> SPNVEACGYSDRVQQITLGNSTITTQEARNAIVCYAEWPEYLSDNDASDVNKTSKPDISVCRFYTLDSKTWKATSKGWCWKLPDALKDMGVFGQNMFYHSLGRTGYTIHVQCNATKFHSGCLLVVVIPEHQLASHEGGTVSVKYKYTHPGDRGIDLDTVEVAGGPTSDAIYNMDGTLLGNLLIFPHQFINMRTNNTATIVVPYINSVPIDSMTRHNNVSLMVVPIAPLNAPTGSSPTLPVTVTIAPMCTEFT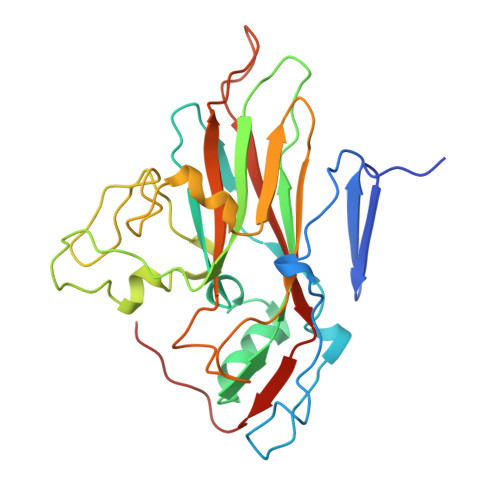GIRSRSIVPQ> VLGKPQTDPTLEWFLSHCHIHKYPSKSTLIHQGEKAETLYYIVKGSVAVLIKDEEGKEMIL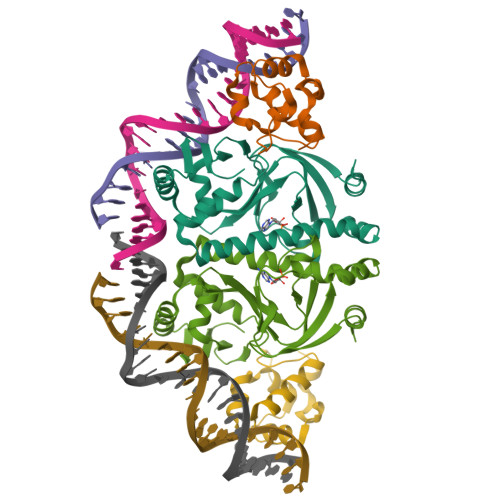SYLNQGDFIGELGLFEEGQERSAWVRAKTACEVAEISYKKFRQLIQVNPDILMRLSAQMARRLQVTSEKVGNLAFLDVTGRIAQTLLNLAKQPDAMTHPDGMQIKITRQEIGQIVGCSRETVGRILKMLEDQNLISAHGKTIVVYGTR;> KPEFDPILLRPVDDLELTVRSANCLKAEAIHYIGDLVQRTEVELLKTPNLGKKSLTEIKDVLASRGLSLGMRLENWPPASIADE>MNVLVIEDDKVFRGLLEEYLSMKGIKVESAERGKEAYKLLSEKHFNVVLLDLLLPDVNGLEILKWIKERSPETEVIVITGHGTIKTAVEAMKMGAYDFLTKPCMLEEIELTINKAIEHRKLRKENELLRREKDLKEEEYVFESPKMKEILEKIKKISCAECPVLITGESGVGKEVVARLIHKLSDRSKEPFVALNVASIPRDIFEAELFGYEKGAFTGAVSSKEGFFELADGGTLFLDEIGELSLEAQAKLLRVIESGKFYRLGGRKEIEVNVRILAATNRNIK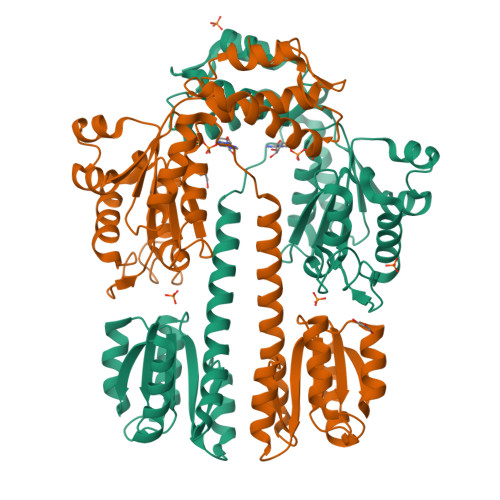ELVKEGKFREDLYYRLGVIEIEIPPLRERKEDIIPLANHFLKKFSRKYAKEVEGFTKSAQELLLSYPWYGNVRELKNVIERAVLFSEGKFIDRGELSCLVNSK[2x]> MAFNFGATTGTPANQGTTGFSLGTFTPKTTTSGFGFGTTTTTAPTGFGGGFGGFGATTTASTGPAFSFTTPANTTSGLFGATQNKGFGFGTGFGSTTTSTGLGTGLGTGLGFTGFNTSQQQQQQSVLGAGLFNQSFQSTPQSNQLINTASALSAPTLLGDERDAILAKWNQLQAFWGTGKGFFMNNTPPVEFTQENPFCRFKAVGFSYIPNNKDEDGLISLIFNKKESDIRGQQQQLVESLHKVLGGHQTLTVNVEGVKTKADNQTEVIIYVVERSPNGTSRRVGASALFSYFEQAHIKANMQQLGVTGAMAQTELSPVQIKQLIQNPLSGVDPIIWEQAKVDNPDPERLIPVPMIGFKELLRRLEVQDQMTKQHQSRLDIISEDIGELQKNQ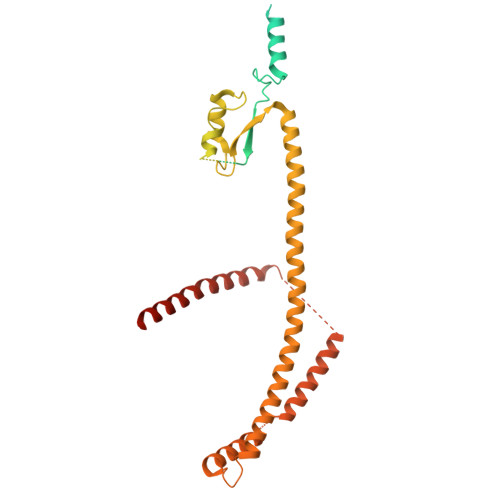TTTMAKIGQYKRKLMELSHRVLQVLIKQEIQRKSGFAIQAEEEQLRVQLDTIQSELNAPTQFKGRLNELMSQIRMQNHFGAVRSEEKYYVDADLLREIKQHLKQQQEGVSHLISIIKDNHEDIKLIEQGLNDNLHMRTGFLS>[4x]MVVTATFAGIDATKHLIGGQWVEGNSDRISTNINPYDDSVIAESKQASIADVDAAYEAAKKAQAEWAATPAAERSAIIYRAAELLEEHREEIVEWLIKESGSTRSKA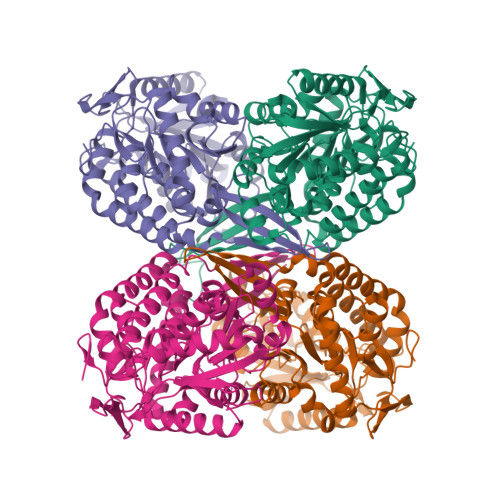NLEITLAGNITKESASFPGRVHGRISPSNTPGKENRVYRVAKGVVGVISPWNFPLNLSIRSVAPALAVGNAVVIKPASDTPVTGGVIPARIFEEAGVPAGVISTVAGAGSEIGDHFVTHAVPKLISFTGSTPVGRRVGELAINGGPMKTVALELGGNAPFVVLADADIDAAAQAAAVGAFLHQGQICMSINRVIVDAAVHDEFLEKFVEAVKNIPTGDPSAEGTLVGPVINDSQLSGLKEKIELAKKEGATVQVEGPIEGRLVHPHVFSDVTSDMEIAREEIFGPLISVLKADDEAHAAELANASDFGLSAAVWSKDIDRAAQFALQIDSGMVHINDLTVNDEPHVMFGGSKNSGLGRFNGDWAIEEFTTDRWIGIKRSAENLYFQSHHHHHHWSHPQFEK> GSHMSRVQLALRVPDL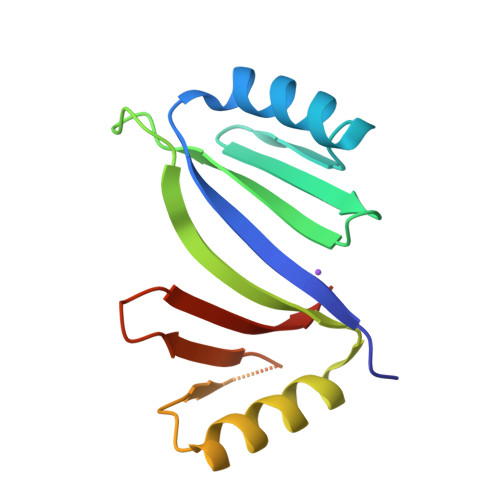EASIGFYSKLFGTGPAKVRPGYANFAIAEPPLKLVLIEGAGEDATRLDHLGVEVEDSAQVGHAARRLKESGLATVEENDTACCYAVQDKVWVTGPGGEPWEVYVVKGDAD> EQLTKCEVFRELKDLKGYGGVSLPEWVCTTFHTSGYDTQAIVQNNDSTEYGLFQINNKIWCKDDQNPHSSNICNISCDKFLDDD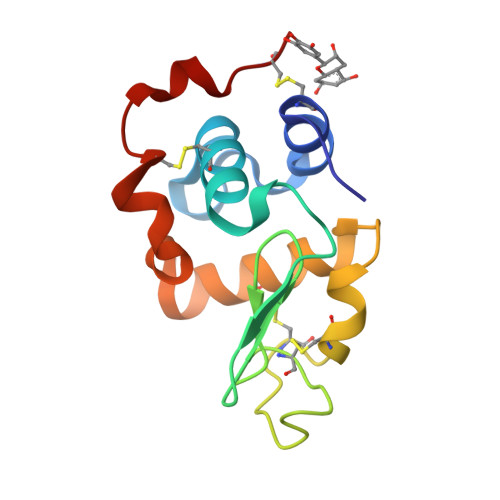LTDDIMCVKKILDKVGINYWLAHKALCSEKLDQWLCE> MSQSNRELVVDFLSYKLSQKGYSWSQFSDVEENRTEAPEGTESEMETPSAINGNPSWHLADSPAVNGATGHSSSLDAREVIPMAAVKQALREAGDEFELRYRRAFSDLTSQLHITPGTAYQSFEQVVNELFRDGVN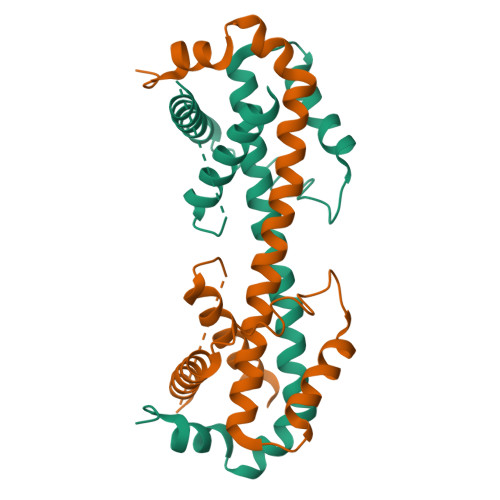WGRIVAFFSFGGALCVESVDKEMQVLVSRIAAWMATYLNDHLEPWIQENGGWDTFVELYGNNAAAESRKGQERFNEHHHHHH>[4x]GGVDREAMARCIEECLRCAQACTACADACLSEPTV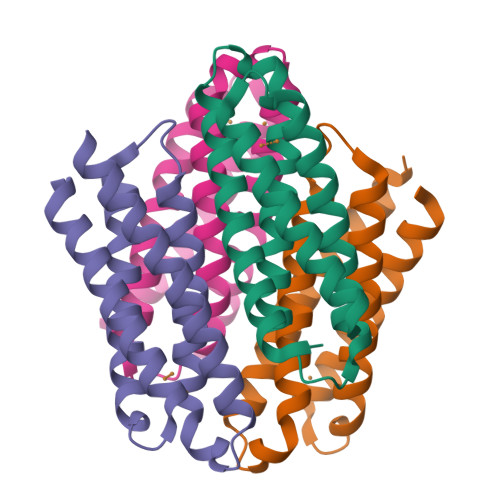ADLTKCIRTDMDCADVCTATAAVLSRHTGYDANVTRAVLQACATVCAACGDECARHAGMHEHCRVCAEACRSCEQACQELLAGLG> SGFNNDPFVQRKLGTSGLNQPTFQQTDLSQVWPEANQHFSKEIDDEANSYFQRIYNHPPHPTMSVDEVLEMLQRFKDSTIKREREVFNCMLRNLFEEYRFFPQYPDKELHITACLFGGIIEKGLVTYMALGLALRYVLEALRKPFGSKMYYFG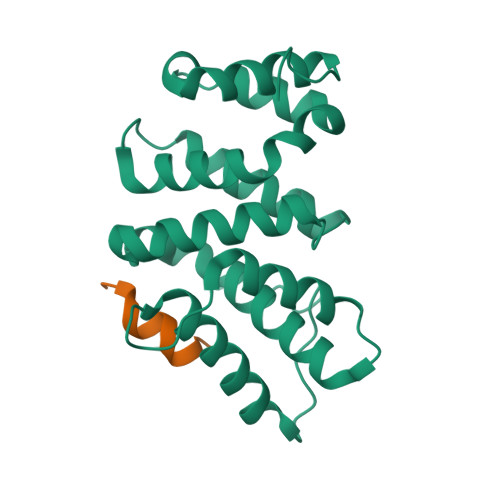IAALDRFKNRLKDYPQYCQHLASISHFMQFPHHLQEYIEYGQQSRDPPVK;> APRRLPIFNRISVSE3-(cyclohexylmethyl)-6,8-bis(oxidanyl)isochromen-1-one 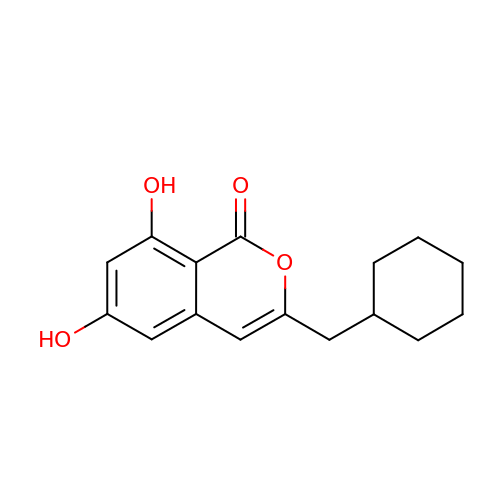| C16 H18 O4 | ZYQPLLMXINVPHW-UHFFFAOYSA-N> TVESNWGGAI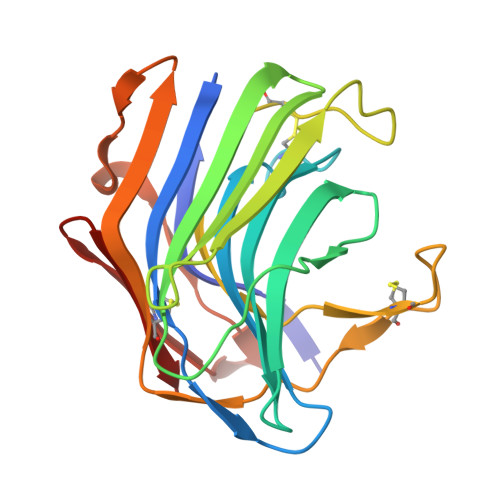LIGSDFDTVSATANVPSASGGSSAAGTAWVGIDGDTCQTAILQTGFDWYGDGTYDAWYEWYPEVSDDFSGITISEGDSIQMSVTATSDTSGSATLENLTTGQKVSKSFSNESSGSLCRTNAEFIIEDFEECNSNGSDCEFVPFASFSPAVEFTDCSVTSDGESVSLDDAQITQVIINNQDVTDCSVSGTTVSCSYV> AQSVPYGVSQIKAPALHSQGYCGSNVKVAVIDSGIDSSHPDLKVAGGASMVPSETN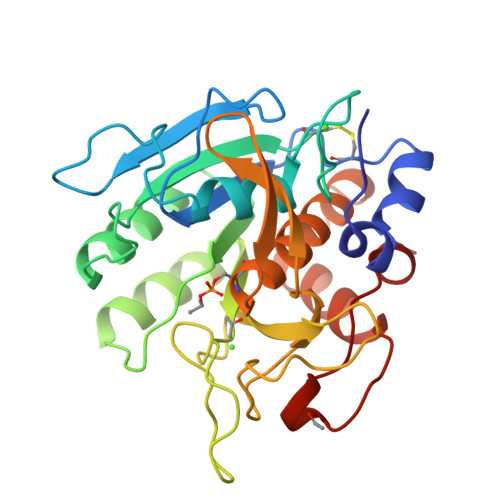PFQDNNSHGTHVAGTVAALNNSIGVLGVAPCASLYAVKVLGADGSGQYSWIINGIEWAIANNMDVINMSLGGPSGSAALKAAVDKAVASGVVVVAAAGNEGTSGSSSTVGYPAKYPSVIAVGAVDSSNQRASFSSVGPELDVMAPGVSIQSTLPGNKYGAYSGTSMASPHVAGAAALILSKHPNWTNTQVRSSLENTTTKLGDSFYYGKGLINVQAAAQ>[2x]MLLHEHGLNTPPAMKDEADQFVVSPTNWAGIIDQALAPPRTRKSYQKSMVSISGTRAVIETRSSKNIMTVDDLMTLFALFTLTVQYHDHHQDDYHFNAKQAPNKTPL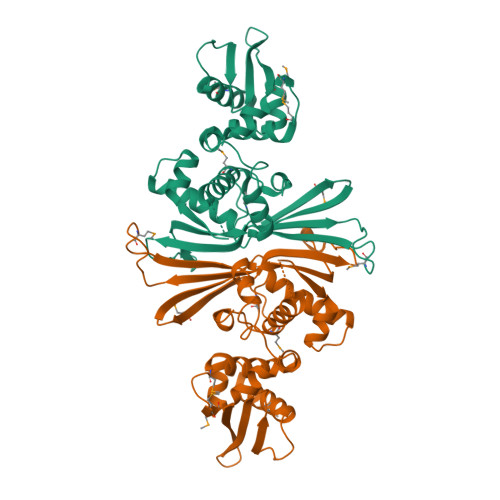YITDILSLRGKKDSGPARDSIRDSIDRIEFTDFQLHELTGRWLSENMPEGFKSDRFRFLARTITASEEAPVEGSDGEIRIKPNLYILVWEPSFFEELLTRDYFFLFPPEILKQHTLVFQLYSYFRSRMSRRHTDVMMLSELNQKLARNIEWRRFSMDLIRELRRLSEGKGSEDLFVVNLWGYHLTVKSIEEKGKVVDYQVDIKCDVEEVLRYSRAKTTNAGKRHHHHHH>[2x]MGHHHHHHENLYFQGHMQNVSLRELAEKLNIYIGFAAINNFWSLSDEEKYMEVARREFNILTPENQMKWDTIHPERDRYNFTPAEKHVEFAEENNMIVHGHTLVWHNQLPGWITGREWTKEELLNVLEDHIKTVVSHFKGRVKIWDVVNEAVS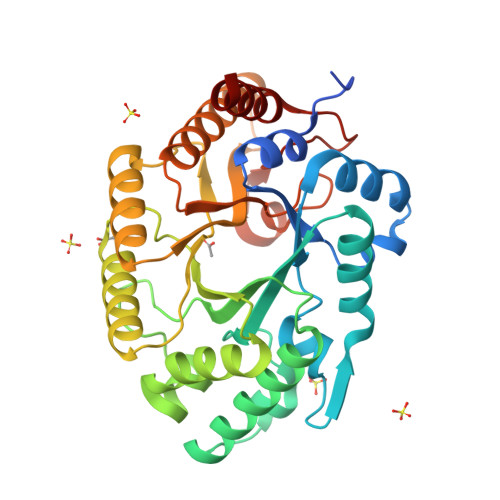DSGTYRESVWYKTIGPEYIEKAFRWTKEADPDAILIYNDYSIEEINAKSNFVYNMIKELKEKGVPVDGIGFQMHIDYRGLNYDSFRRNLERFAKLGLQIYITEMDVRIPLSGSEDYYLKKQAEICAKIFDICLDNPAVKAIQFWGFTDKYSWVPGFFKGYGKALLFDENYNPKPCYYAIKEVLEKKIE> HHHHHHSSGLVPRGSHEVGALQELVVQKGWRLPEYTVTQESGPAHRKEFTMTCRVERFIEIGSGTSKKLA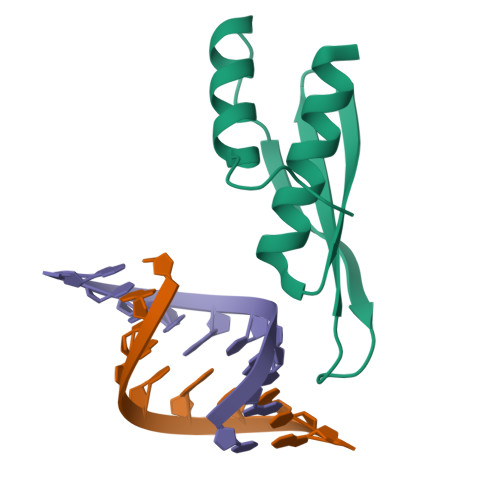KRNAAAKMLLRVHTVPLD> TTPIVHLKGDANTLKCLRYRFKKHCTLYTAVSSTWHWTGHNVKHKSAIVTLTY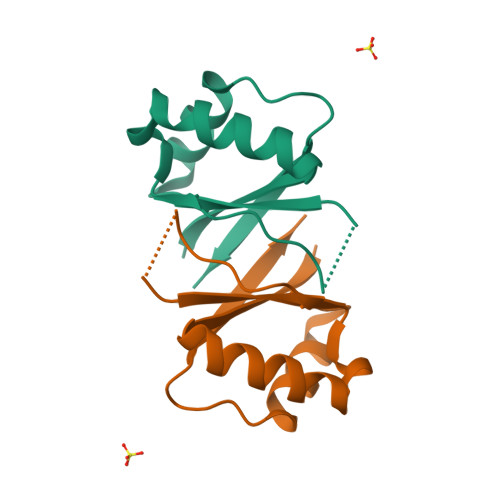DSEWQRDQFLSQVKIPKTITVSTGFMSIGGGTGGGSGGGS>[4x]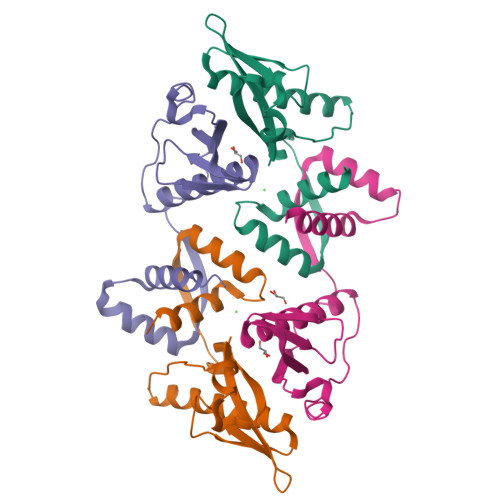MMEFPIAVHKDDGSVYGVTVPDIPGVHSWGETIDDAIKNTREAIVGHVETLIELGEDVEFTCSTVEELVAKPEYAGAVWALVSVDLSQLDSKPERINVSIPRFVLHKIDAYVASRHETRSGFLARAALEALNEGKKHHHHHH>[2x]MVETLPALEIGEDERLDLENLATGAFFPVKGFMTREEALSVAHEMRLPTGEVWTIPILLQFREKPRVGPGNTVALLHGGERVALLHVAEAYELDLEALARAVFGTDSETHPGVARLYGKGPYALAGRVEVLKPRPRTPLEKTPEEVRAFFRQRGWRKVVAFQTRNAPHRAHE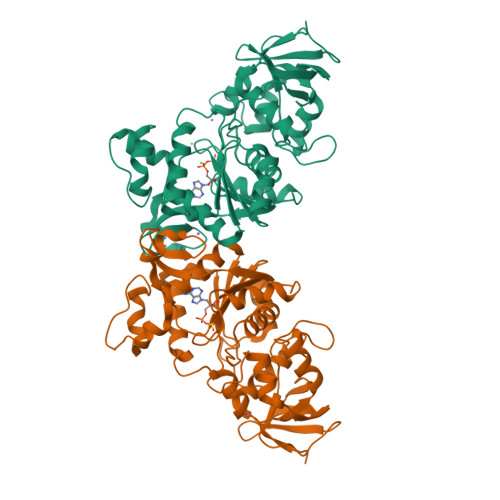YLIRLGLELADGVLVHPILGAKKPDDFPTEVIVEAYQALIRDFLPQERVAFFGLATPMRYAGPKEAVFHALVRKNFGATHFLVGRDHAGVGDFYDPYAAHRIFDRLPPLGIEIVKVGAVFHCPLCGGIASERTCPEGHREKRTAISMTKVRALLREGKAPPSELVRPELLPILRRGV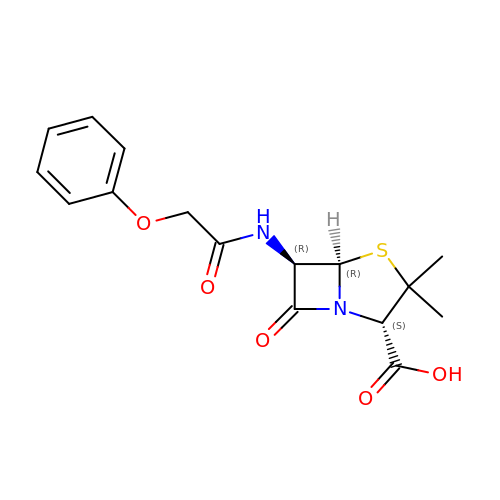(2S,5R,6R)-3,3-DIMETHYL-7-OXO-6-(2-PHENOXYACETAMIDO)-4-THIA-1- AZABICYCLO(3.2.0)HEPTANE-2-CARBOXYLIC ACID | C16 H18 N2 O5 S | BPLBGHOLXOTWMN-MBNYWOFBSA-N3,5-difluoro-L-tyrosine | C9 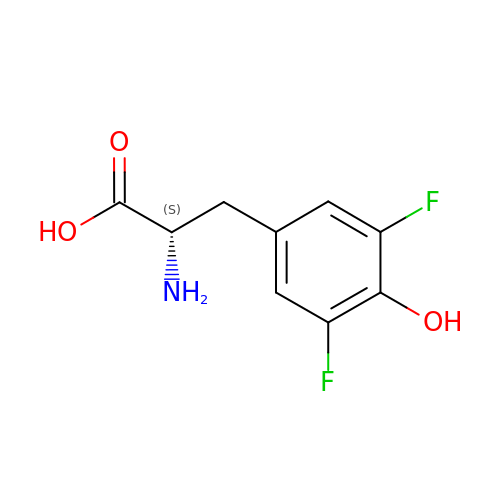H9 F2 N O3 | KPKMCRFCNWVLDA-ZETCQYMHSA-N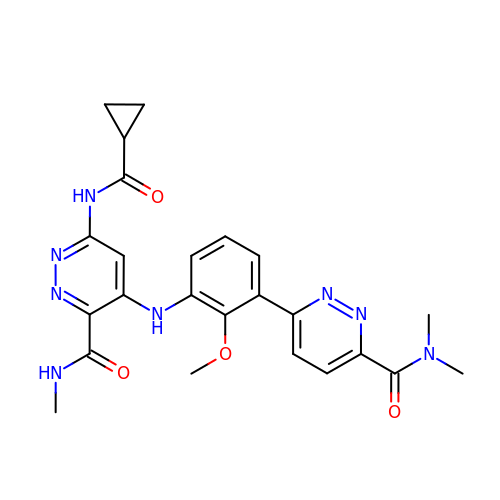6-[(cyclopropanecarbonyl)amino]-4-({3-[6-(dimethylcarbamoyl)pyridazin-3-yl]-2-methoxyphenyl}amino)-N-methylpyridazine-3-carboxamide | C24 H26 N8 O4 | YRGAWFHWYYVABX-UHFFFAOYSA-N Here, we identified the first cytoplasmic membrane-bound phospholipase A1 (PlaF) from Pseudomonas aeruginosa, which might be involved in the Lands cycle. PlaF is an important virulence factor, as the P. aeruginosa ΔplaF mutant showed strongly attenuated virulence in Galleria mellonella and macrophages. PlaF, purified with n-octyl-β-D-glucoside (OG) showed PLA1 but no PLA2 activity toward the artificial substrates specific to each of these two phospholipase families and the natural phospholipid diacyl phosphatidylglycerol containing pentanoic and oleic acid at the sn-1 and sn-2 positions, respectively. PlaF dimerization, mediated solely through the intermolecular interactions of TM and juxtamembrane regions, inhibits its activity.

To gain insights into the PlaF structure, we crystallized the OG-solubilized PlaF protein purified from P. aeruginosa membranes. The structure was refined at a resolution of up to 2.0 Å. The final model in the asymmetric unit consists of two protein molecules (PlaFA and PlaFB), which are related by improper twofold non-crystallographic symmetry. Active site cavities of both the monomers reveal non-covalently bound ligands—myristic acid (MYR), OG, and isopropyl alcohol (IPA) in PlaFA; and undecyclic acid (11A), OG, and IPA in PlaFB. These FAs are the natural ligands from the homologous organism P. aeruginosa that were co-purified with PlaF, as confirmed by gas chromatography-mass spectrometric (GC-MS) analysis of organic solvent extracts of purified PlaF. The N-terminal 38 amino acids form a long, kinked helix that comprises the putative TM (αTM1) and the JM (αJM1) helices, connecting the catalytic domain with the membrane. The TM-JM helices adopt a coiled-coil-like conformation, where the αTM1 crosses its counterpart at V14 to form an elongated X-shaped dimer interface with the buried surface area of 656 Å2 per monomer. The catalytic domain of PlaF adopts a canonical α/β-hydrolase fold (Ollis et al., 1992) with three α-helices forming a distinct lid-like domain that covers the active site. The active site of PlaF comprises the typical serine-hydrolase catalytic triad with S137, D258, and H286 interacting through H-bonds (Jaeger et al., 1994). Finally, the H-bond interaction of catalytic S137 with the carboxyl group of MYR completes an intricate ligand-mediated interaction network bridging the catalytic (S137) and dimerization (V33) sites in PlaF.

>[2x]MKRFLLGLVLLLAVAAGVLYFVPATLLASVRTVERGLAGLSEHSVQVDNLEIAYLEGGSEKNPTLLLIHGFGADKDNWLRFARPLTERYHVVALDLPGFGDSSKPQQASYDVGTQAERVANFAAAIGVRRLHLAGNSMGGHIAALYAARHPEQVLSLALIDNAGVMPARKSELFEDLERGENPLVVRQPEDFQKLLDFVFVQQPPLPAPLKRYLGERAVAASAFNAQIFEQLRQRYIPLEPELPKIEAPTLLLWGDRDRVLDVSSIEVMRPLLKRPSVVIMENCGHVPMVERPEETAQHYQAFLDGVRNAQVAGRGHHHHHH> MDVDLFKLSLDDTSSVKGSLLDTRFAQVRVVIPKAMAGGNELLNSNLYDILVVDNNFRAAAALAHTHIIEGQIKCVCTINLPENTGCCLALCVNSSNRGQFSTDIYTIGSQDRMLWNPAC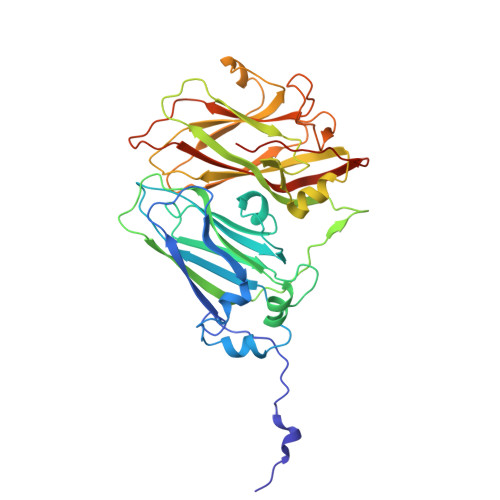SKNSTFTFNPNPCGTGWSLEFLRRTKFHISVVCVSGWSAQPQTDLVMTMDFFVANVPCVPRIYNLGSPGQTLWLNRWMGKLSFGQGVSNDIKSMPLAIGGGAGAKDSILMNMTNAYLSLWRYFHGDLVFEVNKMSSPYIKSTVTFFIGFGGVSFQPELEDFPNKLVQFSEVQEKIELKFTRAEFLTAWSTQVDPAAQLANDGCPYLYAMVHDSTASTIVGDFNLGVTLTRIENFAGIGCNPGIQGARLLGSAIATPQ AMINO-CASTANOSPERMINE | C8 H16 N2 O3 | 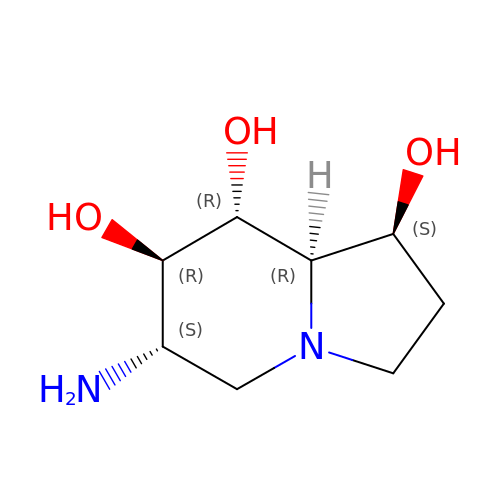LKBIVYWSUHFIBP-TVNFTVLESA-N The 169 rhinovirus (RV) types identified to date are a main cause of the common cold. In many RV types, a ‘pocket factor’, in most cases a myristate, was identified in a hydrophobic pocket lined by amino acid residues mainly contributed by VP1. During infection, the native virus expands and releases the pocket factor and VP4 giving rise to the ‘A particle’.

Incubation in the acidic buffers for one hour at 4 °C followed by neutralisation resulted in the respective formation of non-infectious A particles (in Na+) and a non-infectious novel uncoating intermediate (in K+), which we termed ‘E0 particle’. Incubation of RV-A2 in KPB at pH 5.8 revealed a novel uncoating intermediate (the E0 particle) with a slightly expanded shell and less permeability to PTA than the A particle. Cryo-EM image reconstruction of the E0 particle showed clear differences between A and E0 particles; like native virus, E0 contained VP4 and a pocket factor. Furthermore, the presence of the pocket factor prevented the side chain of MET1193 from moving into the pocket, as is seen in RV-A89 devoid of the pocket factor. Inside the capsid, the genomic RNA is still fully retained and densely packed in the E0 particle. However, the capsid interior shows a bulk density consistent with tightly packed RNA, similar to the native virion. Importantly, no RNA strands are seen protruding or organizing into distinct helices in the E0 map, implying that the genome has not begun to exit. Of note, whereas in the A particle several contacts between RNA and the inner wall of the capsid are seen, in the E0 particle only the stacking interactions of the RNA with aromatic residues are clearly discernible. Therefore, E0 particles likely mark an abortive branch of the entry pathway that might function as a host-defence.

> NPVENYIDEVLNEVLVVPNINSSNPTTSNSAPALDAAETGHTSSVQPEDVIETRYVQTSQTRDEMSLESFLGRSGCIHESKLEVTLANYNKENFTVWAINLQEMAQIRRKFELFTYTRFDSEITLVPCISALSQDIGHITMQYMYVPPGAPVPNSRDDYAWQSGTNASVFWQHGQAYPRFSLPFLSVASAYYMFYDGYDEQDQNYGTANTNNMGSLCSRIVTEKHIHKVHIMTRIYHKAKHVKAWCPRPPRALEYTRAHRTNFKIEDRSIQTAIVTRPIITTA;> SPTVEACGYSDRIIQITRGDSTITSQDVANAIVAYGVWPHYLSSKDASAIDKPSQPDTSSNRFYTLRSVTWSSSSKGWWWKLPDALKDMGIFGENMFYHYLGRSGYTIHVQCNASKFHQGTLIVALIPEHQIASALHGNVNVGYNYTHPGETGREVKAETRLNPDLQPTEEYWLNFDGTLLGNITIFPHQFINLRSNNSATIIAPYVNAVPMDSMRSHNNWSLVIIPICPLETSSAINTIPITISISPMCAEFSGARAKRQ;> GLPVFITPGSGQFLTTDDFQSPCALPWYHPTKEISIPGEVKNLVEICQVDSLVPINNTDTYINSENMYSVVLQSSINAPDKIFSIRTDVASQPLATTLIGEISSYFTHWTGSLRFSFMFCGTANTTVKLLLAYTPPGIAEPTTRKDAMLGTHVIWDVGLQSTISMVVPWISASHYRNTSPGRSTSGYITCWYQTRLVIPPQTPPTARLLCFVSGCKDFCLRMARDTNLHLQSGAIAQ;> GAQVSRQNVGTHSTQNSVSNGSSLNYFNINYFKDAASNGASKLEFTQDPSKFTDPVKDVLEKGIPTLQ>AQQGVFTLPARINFGVTVLVNSAATQHVEIFVDNEPRAAFSGVGTGDNNLGTKVINSGSGNVRVQITANGRQSDLVSSQLVLANKLNLAVVGSED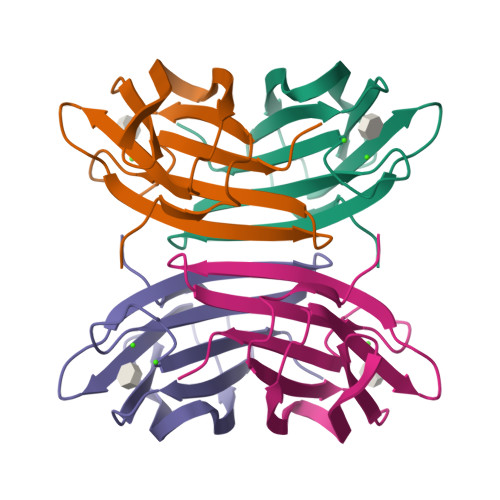GTDMDYNDSIVILNWPLG[2x]> DVPQWEV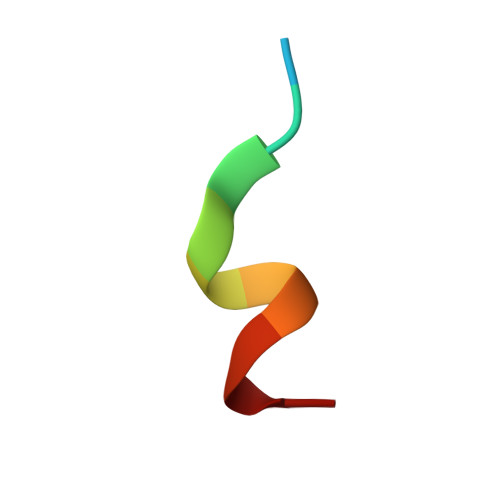FFKR> GSQTNTGEIYFVELVKEDGTLGFSVTGGINTSVPHGGIYVKSIIPGGPAAKEGQILQGDRLLQVDGVSLCGLTHKQAVQCLKGPGQVARLVLE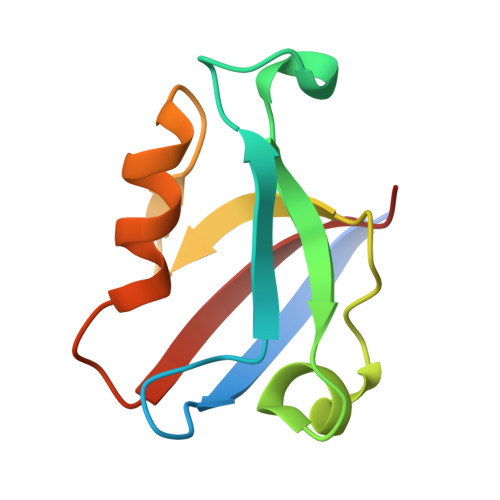RRG>AVPETRPNHTIYINNLNEKIKKDELKKSLHAIFSRFGQILDI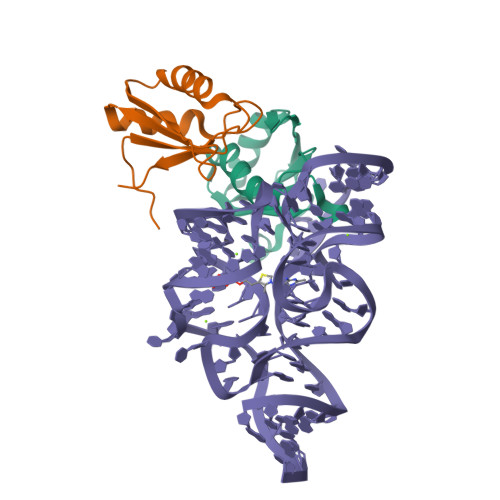LVSRSLKMRGQAFVIFKEVSSATNALRSMQGFPFYDKPMRIQYAKTDSDIIAKM[4x]>[2x]MSLKTLDGKITRPTSDKVRGAIFNMIGPYFNG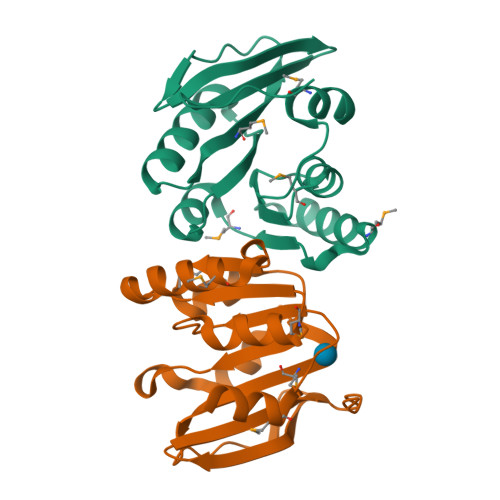GRVLDLFAGSGGLAIEAVSRGMSAAVLVEKNRKAQAIIQDNIIMTKAENRFTLLKMEAERAIDCLTGRFDLVFLDPPYAKETIVATIEALAAKNLLSEQVMVVCETDKTVLLPKEIATLGIWKEKIYGISKVTVYVNEGHHHHHH cyclopropylmethanamine | C4 H9 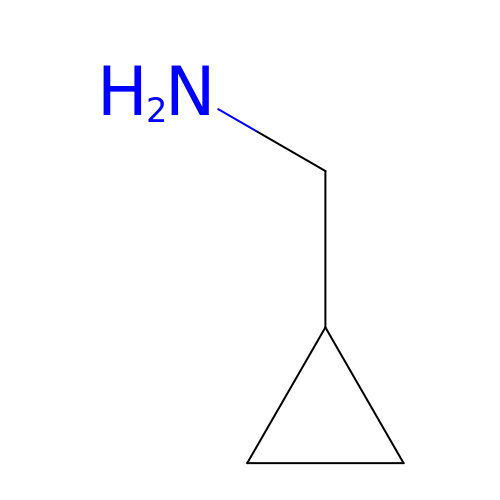N | IGSKHXTUVXSOMB-UHFFFAOYSA-N> ADTLDNVNLVSSPVHSGFLVSFMVDARGGSMRGSRHHGM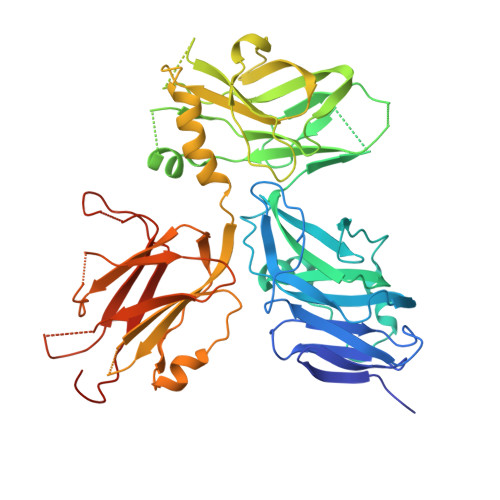RIIIPPRKCTAPTRITCRLVKRHKLANPPPMVEGEGLASRLVEMGPAGAQFLGPVIVEIPHFGSMRGKERELIVLRSENGETWKEHQFDSKNEDLSELLNGMDEELDSPEELGTKRICRIITKDFPQYFAVVSRIKQESNQIGPEGGILSSTTVPLVQASFPEGALTKRIRVGLQAQPVPEETVKKILGNKATFSPIVTVEPRRRKFHKPITMTIPVPPPSGEGVSNGYKGDTTPSLRLLCSITGGTSPAQWEDITGTTPLTFIKDCVSFTTNVSARFWLADCHQVLETVGLASQLYRELICVPYMAKFVVFAKTNDPVESSLRCFCMTDDRVDKTLEQQENFEEVARSKDIEVLEGKPIYVDCYGNLAPLTKGGQQLVFNFYSFKENRLPFSIKVRDTSQEPCGRLSFLKEPKTTKGLPQTAVCNLNITLPAHKKAEKADRRQSFTSLALR>MTTLADVKKRIGLKDEKQDEQLEEIIKSCESQLLSMLPIEVEQIPERFSYMIKEVAVKRYNRIGAEGMTSEAVDGRSNAYELNDFKEYEAIIDNYFNARTRTKKGRAVFF[2x];> MRYEDRVIFQLEQVATYNPKTSKKENTLITYDAIPCNINPISRARKQLEFGDVKNDVSVLRIKESISYPVSHVLVNGIRYKIVDTRIYRHETSYYIEEVN;> MTPNLQLYNKAYETLQGYGFPVISRKEMQQEIPYPFFVIKMPESNRSKYTFDSYSGDTNLVIDIWSVSDDLGHHDGLVKRCIDDLTPSVKTNDYDFEEDDTNITQLVDDTTNQELLHTSITISYKTF;>[2x]MANMKNSNDRIILFRKAGEKVDATKMLFLTEYGLSHEADTDTEDTMDGSYNTGGSVESTMSGTAKMFYGDDFADEIEDAVVDRVLYEAWEVESRIPGKNGDSAKFKAKYFQGFHNKFELKAEANGIDEYEYEYGVNGRFQRGFATLPEA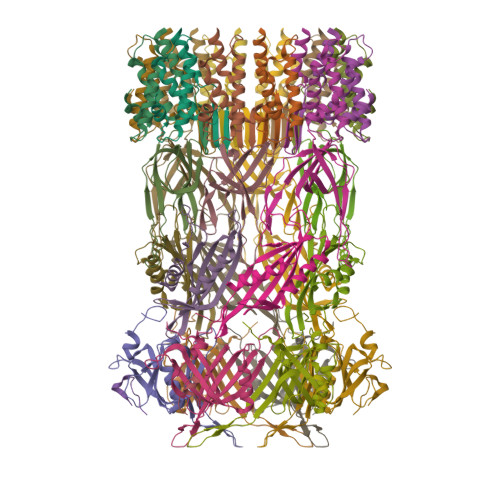VTKKLKATGYRFHDTTKEDALTSEDLTAIPQPKVDSSTVTPGEV> MRLSLLRRFCEYVPKGAPTQVSLSVETPYGVTRAFRMTEMAAAAADAERDAKGFFYLPRMDYDVGQGV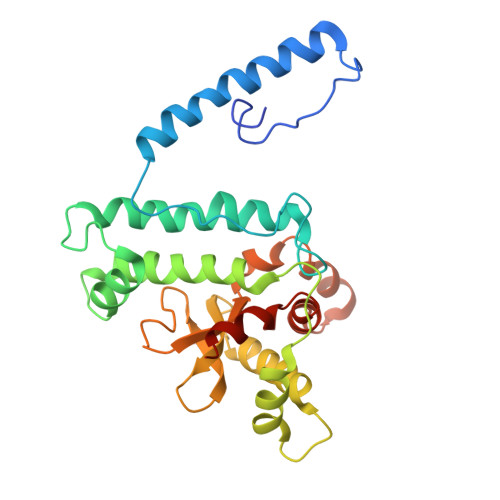APLMSRKQFDVQYNVFHKAAVDRLNAHTLGSELEGHNLNVVIRNSSFDASHAVIHAAASEHFNYCFWYRSLRPWGTAVPARLKEELQLQYSQNGTLDAVKEVQRLFTVAALSQQSAGGWVYLVWTGKAFDVIPFDHGTCPIGSDLIPLLALNTHESARCYDYPLAAEDEEGDEVERFVRNFFKTCNWRLVEHYFLQCGRA>GLTYSQTMELKDSMLQLDPNAKTWIDIEGRPEDPVEIAIYQ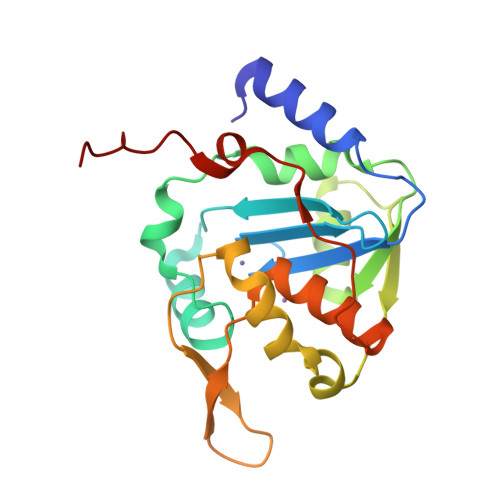PNNGQYIHFYREPTDIKQFKQDSKHSHGIDIQDLFSVQPGLTSAVIESLPKNMVLSCQGADDIRKLLDSQNRRDIKLIDVSMQKDDARKFEDKIWDEYKHLCRMHTGIVTQKKKRGGKEEVTPHCALLDCLMFEAAVIGSPQIPTPRPVLSRDLVFRTGPPRVVL[3x]>MAHHHHHHMGRLIIVSNRVAPISEGGPAAGGLAVGVYDALKETGGMWFGWSGDVLSSGQPQIKVEERGPVTFATIALMRRDYDQYYRGFSNATLWPAFHYRADLLQYDRHDFEGYWRVNAWLAQQLVPLLREDDVIWVHDYHLIPFAQALRAAGVKNRIGFFLHIPFPASQVLLAVPPHRELVEALCSFDLLGFQTAPDLRAFCDYIVNEANGTADPSASGPLTIHAFGRTLRAAAYPIGVYPDEIAELAKAGERGKPVRTMKATLHSRKLIMSVDRLDYSKGLVERFRAFERLLEHSTAQRNKVSFLQIAPPTRADMHAYQDIRLQLEGESGRINGRFAELDWTPILYIHKQYERSVLAALFRTAHVGYVTPLRDGMNLVAKEYVSAQDPENPGVLVLSRFAGAAQELDGALIVNPVDIDGMAEALARALDMPLAERQARHRDMMVQLRENNVSVWRDNFMRDLQGVAGAKGTRNGKARAVAGKKAARETQAG[8x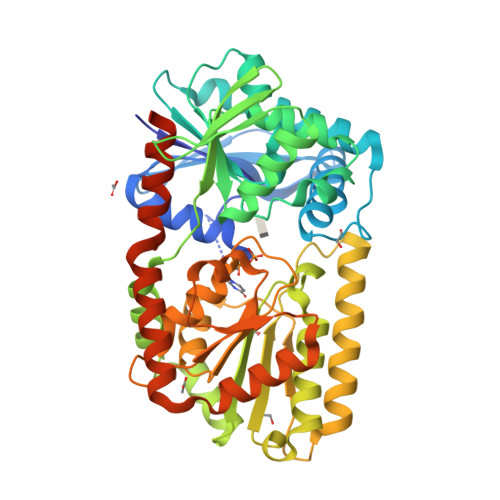]> GSDKRGPQSAEPDPLERLEVKKVQQQHENEKDDSGRDTKSGGKVAKAMTKGDTIAGKLLTTPSRLFKLLIPLTTINR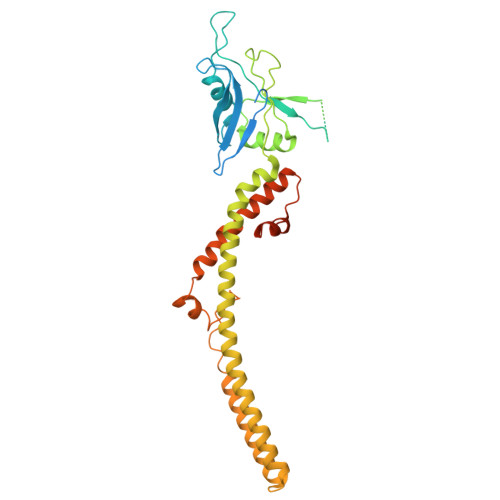KDIEQIAILIHPQQPLSHLERLIQSEVPPIEDENGQKRPPFVSFIALQLEQDAIRPKRGMYEGTDAEIHRVEGGKDDATVAKRGEDFQEVDETFSYLRRPGPGQGDKEQRFIRWSQSTEIGDFIRDAARAKEFIVTIEGAPAGLEQIHVAVPSFDERTYFLRMRLRKISRRIQGLAEIKHECDALAHRGAQRVALGGFGILAFWWYIVYKLTFETDLGWDTMEPVTYLVSLSTLMGGYLWFLYHNREISYRSALDFTINARQKKLYQMKGIDLQVWESLIDEANAIRREIKNIAAEYDVDWDERKDEQDDRVTEALKKERRLKNGSQKEERPKDDRDDD> GSPELRQEHQQLAQEFQQLLQEIQQLGRELLKGELQGIKQLREASEKARNPEKKSVLQKILEDEEKHIELHETLQQTGQEAQQLLQELQQTGQELWQLGGSGGPELRQKHQQLAQKIQQLLQKHQQLGAKILEDEEKHIELLETILGGSGGDELRELLKGELQGIKQYRELQQLGQKAQQLVQKLQQTGQKLWQLG

Here, we report the rational design, X-ray crystal structure, and electron transfer activity of a multi-cofactor protein that incorporates essential elements of photosynthetic reaction centers. To this end, we have designed a photosynthetic reaction center protein maquette (the RC maquette) and solved its X-ray crystal structure in multiple states of assembly. To begin reverse-engineering photosynthetic reaction centers, we use first principles of protein folding to construct a single-chain framework for positioning DPA cofactors that consists of an extended four α-helix bundle coiled-coil. The RC maquette uses histidine (His) residues in the hydrophobic core to coordinate the central metals of tetrapyrroles for site-specific cofactor binding.

Hydrophobic core packing, rotameric states of heme-ligating histidines, and second shell histidine-threonine hydrogen bonds are similar to the cytochrome b subunit of cytochromes bc1 and b6f. Even the orientation of the maquette heme relative to the superhelical bundle axis is conspicuously similar, suggesting that the particular conformation of heme in the natural proteins is not precisely controlled for any functional purpose, but rather follows directly from structural constraints demanded by this protein fold. In the nearby metal binding site, Glu/His ligation of Cd(II) in the RC maquette accurately reproduces the geometry of the binuclear Mn(II) cluster shown to be photochemically active in modified bacterioferritin. At neutral pH, Zn(II) and Cd(II) suppress Tyr oxidation. These metals may electrostatically inhibit proton transfer from Tyr to protonatable residues in the metal cluster site. While the introduction of a hydrogen bond from Tyr to a His residue appears to have little impact on the lifetime or yield of charge separation by itself, the addition of Asp31 adjacent to the His71-Tyr168 hydrogen bond raises the yield from 2 ± 1% to 11.5 ± 0.7% and shortens the lifetime of charge separation from 40 ± 20 ms to 3 ± 1 ms at pH 9.5. Without a crystal structure of the L31D/L71H RC maquette mutant, however, we cannot confirm that the Asp31-His71 hydrogen bond forms; it remains possible that Asp31 raises the quantum yield of electron transfer by altering the dynamics and hydration of Tyr168 rather than by acting directly as a proton acceptor for His71. Bacterioferritin-like ferroxidase activity demonstrates that the diiron site is redox active. Light-induced electron transfer is clear as near-stoichiometric Fe(II) prolongs the lifetime of charge separation from 2.0 ms to 250 ms at pH 7.5 in RC maquette variant L71H (orange and Supplementary Figs. 8b and 10a).> GGIQMPVFHTRTIESILEPVAQQISHLVIMHEEGEVDGKAIPDLTAPVSAVQAAVSNLVRVGKETVQTTEDQILKRDMPPAFIKVENACTK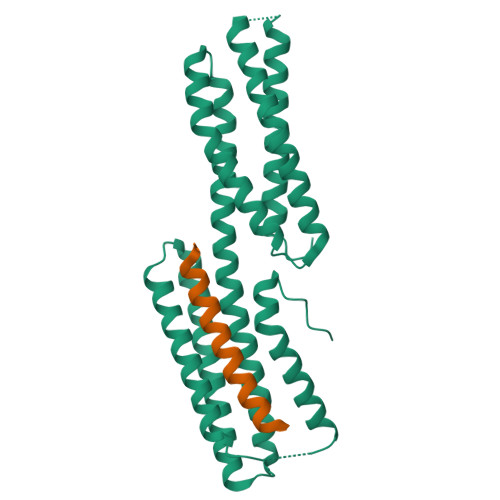LVRAAQMLQADPYSVPARDYLIDGSRGILSGTSDLLLTFDEAEVRKIIRVCKGILEYLTVAEVVETMEDLVTYTKNLGPGMTKMAKMIDERQQELTHQEHRVMLVNSMNTVKELLPVLISAMKIFVTTKNTKSQGIEEALKNRNFTVEKMSAEINEIIRVLQLTSWDEDAWA;> GGIQDSSCTRDDRRERIVAECNAVRQALQDLLSEYMGNAG> GPPPRFQRDFVDLRTDCPSTHPPIRVMQWNILAQALGEGKDNFVQCPVEALKWEERKCLILEEILAYQPDILCLQEVDHYFDTFQPLLSRLGYQGTFFPKPWSPCLDVEHNNGPDGCALFFLQNRFKLVNSANIRLTAMTLKTNQVAIAQTLECKESGRQFCIAVTHLKARTGWERFRSAQGCDLLQNLQ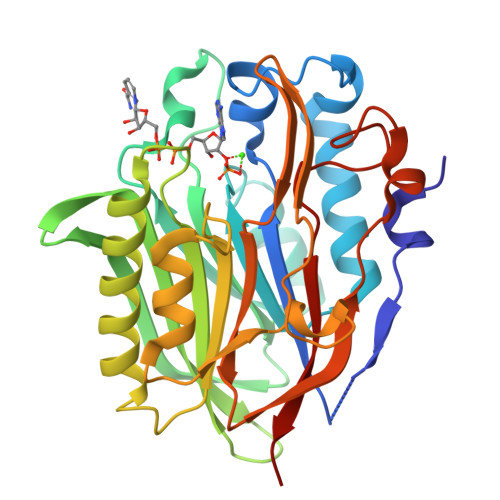NITQGAKIPLIVCGDFNAEPTEEVYKHFASSSLNLNSAYKLLSADGQSEPPYTTWKIRTSGECRHTLDYIWYSKHALNVRSALDLLTEEQIGPNRLPSFNYPSDHLSLVCDFSFTEESDGLS>SKSSHTLKTANSYTDVTVSNSTKKAIRESNQYTDHKFHQLDNRLDKLDTRVDK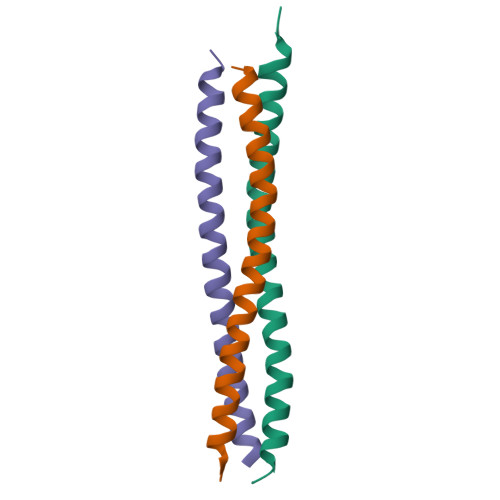GLASSAALNSL[6x]>[2x]STDISTVASPLFEGTEGCFLLYDASTNAEIAQFNKAKCATQMAPDSTFKIALSLMAFDAEIIDQKTIFKWDKTP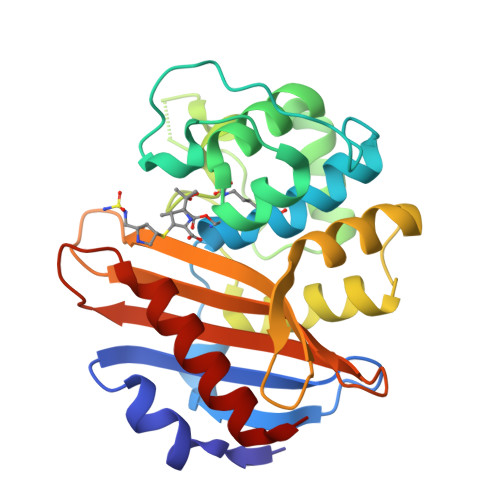KGMEIWNSNHTPKTWMQFSVVWVSQEITQKIGLNKIKNYLKDFDYGNQDFSGDKERNNGLTEAWLESSLKISPEEQIQFLRKIINHNLPVKNSAIENTIENMYLQDLDNSTKLYGKTGAGFTANRTLQNGWFEGFIISKSGHKYVFVSALTGNLGSNLTSSIKAKKNAITILNTLNL Rv0315 is a secreted protein of Mtb, and the signal peptide is cleaved by a signal peptidase before the mature protein is released. Rv0315 can induce dendritic cell (DC) maturation and activation via the activation of MAPK and NF-κB signaling, and it participates in adaptive immunity by inducing T cell immune responses toward T-helper 1 (Th1) polarization via antigen-presenting DCs23. The overall structure of Rv0315 reveals that the protein adopts a sandwich-like β-jelly-roll fold, formed by the face-to-face packing of two antiparallel sheets, which is typical of GH16 enzymes. However, our enzymatic activity assay showed that Rv0315 is actually an inactive β-glucanase that is ineffective for the degradation of 1,3-β-glucans, such as laminarin, and has no activity toward 1,3–1,4-β-glucans, such as β-D-glucan from barley.

The crystal is monoclinic (C121), and its asymmetric unit contains two chains of Rv0315 (designated as chains A and B), and a total of 681 water molecules. Each monomer is composed of 241 amino acids (54–294). The final model of Rv0315 has been refined to Rwork of 18.4% and Rfree of 21.4%. The overall structure comprises 16 β-strands forming two twisted β-sheets, two short a-helices and one calcium ion. The calcium ion binding site is well conserved in GH16 enzymes and has been suggested to be important for protein stability. The β-sheets twist and bend, forming a substrate binding concavity. Two conserved glutamates in the pattern EXDX(X)E are catalytic residues28 in the GH16 family proteins; in Rv0315, Glu-171 is equivalent to the catalytic nucleophile, whereas Glu-176 is the general acid-base catalyst. Rv0315 has a larger cavity than that of the ZgLamAGH16 structure; this large cavity is not present in other known structures of the GH16 family laminarinases. All of these residues related to subsites −2 and −3 were not conserved in Rv0315 and could not form any direct interactions with the substrate. Given all of these differences, polysaccharides may not be able to firmly bind to the cleft of Rv0315 because of its large cavity and the lack of key residues to fix the β-glucans, leading to a lack of detectable catalytic activity for Rv0315.

>MLMPEMDRRRMMMMAGFGALAAALPAPTAWADPSRPAAPAGPTPAPAAPAAATGGLLFHDEFDGPAGSVPDPSKWQVSNHRTPIKNPVGFDRPQFFGQYRDSRQNVFLDGNSNLVLRATREGNRYFGGLVHGLWRGGIGTTWEARIKFNCLAPGMWPAWWLSNDDPGRSGEIDLIEWYGNGTWPSGTTVHANPDGTAFETCPIGVDGGWHNWRVTWNPSGMYFWLDYADGIEPYFSVPATGIEDLNEPIREWPFNDPGYKVFPVLNLAVGGSGGGDPATGSYPQEMLVDWVRVFGSHHHHHH[2x]>[4x]GPMTADAPAGTLAQPGGISDPNLIKLVNKLQDVFTTVGVNNPIDLPQIVVVGSQSSGKSSVLENIVGRDFLPRGQGIVTRRPLVLQLINRQSSGNANGFDERLADSTDKAANLDEWGEFLHLPGQKFYDFNKIRDEINRETEAKVGRNAGISPAPINLRIYSPHVLNLTLVDLPGLTRVPVGDQPRDIERQIRDMILKYIQKPNAIILAVTAANVDLANSDGLKLAREVDPEGQRTIGVLT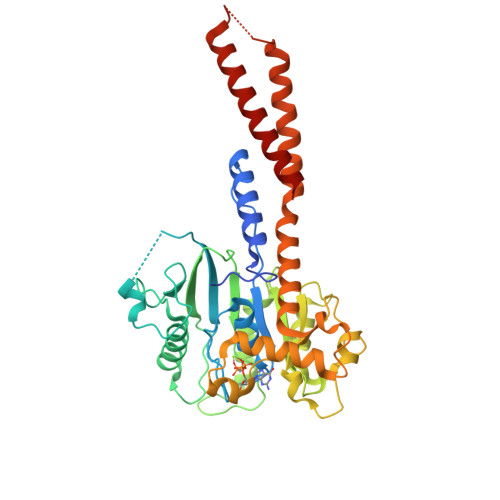KVDLMDEGTDVVDILAGRIIPLRLGYVPVVNRGQRDIDNKKPITAALEAEKAFFENHKAYRNKSAYCGTPYLARKLNLILMMHIKQTLPDIKQRISSSLQKYQQELEALGPSLLGAGAGAESDYTVRRRKECQQMVESLQRAAEIVSQVQ[3-HYDROXY-2-METHYL-5-PHOSPHONOOXYMETHYL-PYRIDIN-4-YLMETHYL]-L-TRYPTOPHANE | C19 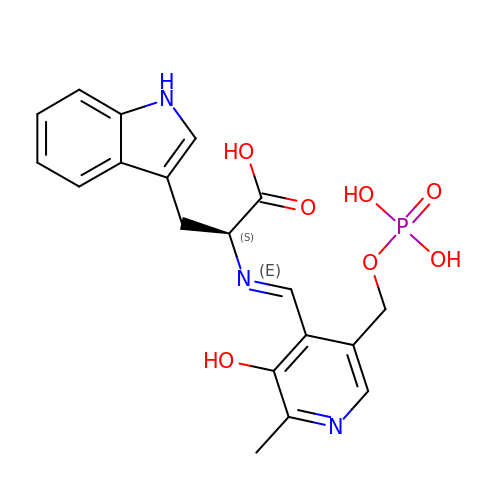H20 N3 O7 P | MFRRQHVPLFTBMS-NUYDQDRBSA-N> MNNPAIQRIEDHIVKSPEDKREYRGLELANGIKVLLISDPTTDKSSAALDVHIGSLSDPPNIPGLSHFCEHMLFLGTKKYPKENEYSQFLSEHAGSSNAFTSGEHTNYYFDVSHEHLEGALDRFAQFFLCPLFDASCKDREVNAVDSEHEKNVMNDAWRLFQLEKATGNPKHPFSKFGTGNKYTLETRPNQEGIDVREELLKFHSTYYSSNLMAICVLGRESLDDLTNLVVKLFSEVENKNVPLPEFPEHPFQEEHLKQLYKIVPIKDIRNLYVTFPIPDLQQYYKSNPGHYLGHLIGHEGPGSLLSELKSKGWVNTLVGGQKEGARGFMFFIINVDLTEEGLLHVEDIILHMFQYIQKLRAEGPQEWVFQECKDLNAVAFRFKDKERPRGYTSKIAGKLHYYPLNGVLTAEYLLEEFRPDLIDMVLDKLRPENVRVAIVSKSFEGKTDRTEQWYGTQYKQEAIPEDVIQKWQNADLNGKFKLPTKNEFIPTNFEILALEKDATPYPALIKDTAMSKLWFKQDDKFFLPKACLNFEFFSPFAYVDPLHCNMAYLYLELLKDSLNEYAYAAELAGLSYDLQNTIYGMYLSVKGYNDKQPILLKKITEKMATFEIDKKRFEIIKEAYMRSLNNFRAEQPHQHAMYYLRLLMTEVAWTKDELKEALDDVTLPRLKAFIPQLLSRLHIEALLHGNITKQAALGVMQMVEDTLIEHAHTKPLLPSQLVRYREVQLPDRGWFVYQRRNEVHNNCGIEIYYQTDMQSTSENMFLELFCQIISEPCFNTLRTKEQLGYIVFSGPRRANGIQGLRFIIQSEKPPHYLESRVEAFLITMEKAIEDMTEEAFQKHIQALAIRRLDKPKKLSAECAKYWGEII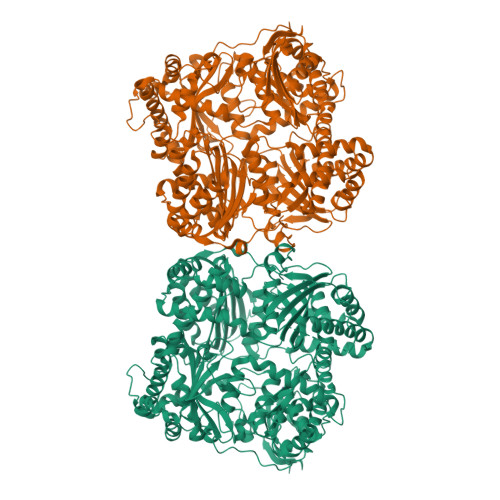SQQYNYDRDNIEVAYLKTLSKDDIIKFYKEMLAVDAPRRHKVSVHVLAREMDSCPVVGEFPSQNDINLSEAPPLPQPEVIHNMTEFKRGLPLFPLVKPHINFMAAKL>[2x]ANPLYQKHIISINDLSRDDLNLVLATAAKLKANPQPELLKHKVIASCFFEASTRTRLSFQTSMHRLGASVVGFSDSANTSLGKKGETLADTISVISTYVDAIVMRHPQEGAARLATEFSGNVPVLNAGDGSNQHPTQTLLDLFTIQQTEGRLDNLHVAMVGDLKYGRTVHSLTQA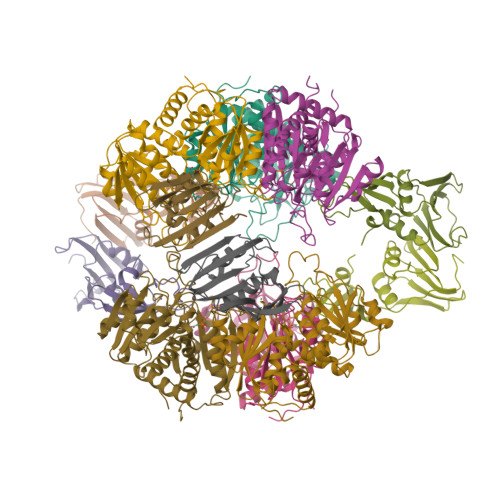LAKFDGNRFYFIAPDALAMPEYILDMLDEKGIAWSLHSSIEEVMAEVDILYMTRVQKERLDPSEYANVKAQFVLRASDLHNAKANMKVLHPLPRVDEIATDVDKTPHAWYFQQAGNGIFARQALLALVLNRDLVL;>[2x]MTHDNKLGVEAIKRGTVIDHIPAQIGFKLLSLFKLTETDQRITIGLNLPSGEMGRKDLIKIENTFLSEDQVDQLALYAPQATVNRIDNYEVVGKSRPSLPERIDNVLVCPNSNCISHAEPVSSSFAVRKRANDIALKCKYCEKEFSHNVVLAN>MNHKVHHHHHHMGGGSTPLPLPQQQPPQQEPPPPPVPLASRAACEALKDGNGDMVWPNAATVVEVAAWRDAAPATASAAALPEHCEVSGAIAKRTGIDGYPYEIKF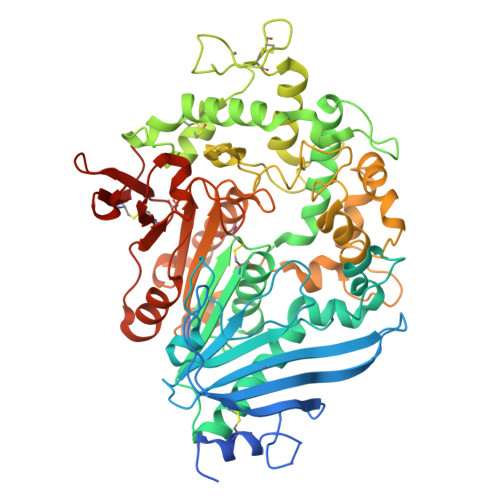RLRMPAEWNGRFFMEGGSGTNGSLSAATGSIGGGQIASALSRNFATIATDGGHDNAVNDNPDALGTVAFGLDPQARLDMGYNSYDQVTQAGKAAVARFYGRAADKSYFIGCSEGGREGMMLSQRFPSHYDGIVAGAPGYQLPKAGISGAWTTQSLAPAAVGLDAQGVPLINKSFSDADLHLLSQAILGTCDALDGLADGIVDNYRACQAAFDPATAANPANGQALQCVGAKTADCLSPVQVTAIKRAMAGPVNSAGTPLYNRWAWDAGMSGLSGTTYNQGWRSWWLGSFNSSANNAQRVSGFSARSWLVDFATPPEPMPMTQVAARMMKFDFDIDPLKIWATSGQFTQSSMDWHGATSTDLAAFRDRGGKMILYHGMSDAAFSALDTADYYERLGAAMPGAAGFARLFLVPGMNHCSGGPGTDRFDMLTPLVAWVERGEAPDQISAWSGTPGYFGVAARTRPLCPYPQIARYKGSGDINTEANFACAAPP[10x]>[4x]SNAMEPVSSWGNTSLVSVDPEIHDLIEKEKRRQCRGIELIASENFTSFAVIEALGSALTNKYSEGIPGNRYYGGNEFIDEIENLCRSRALEAFHCDPAAWGVNVQPYSGSPANFAAYTALLQPHDRIMGLDLPSGGHLTHGYYTSGGKKISATSIYFESLPYKVNFTTGYIDYDKLEEKALDFRPKLLICGGSAYPRDWDYARFRAIADKVGALLLCDMAHISGLVAAQEAANPFEYCDVVTTTTHKSLRGPRAGMIFYRKGPKPPKKGQPEGAVYDFEDKINFAVFPALQGGPHNHQIGALAVALKQANTPGFKVYAKQVKANAVALGNYLMSKGYQIVTNGTENHLVLWDLRPLGLTGNKVEKLCDLCSITLNKNAVFGDSSALAPGGVRIGAPAMTSRGLVEKDFEQIGEFLSRAVTLTLDIQKTYGKLLKDFNKGLVNNKDLDQLKADVEKFSASYEMPGFLMSEMKYKD

Serine hydroxymethyltransferase (SHMT) reversibly interconverts serine and tetrahydrofolate (THF) into glycine and 5,10-methylene-THF (5,10-meTHF). Next, we have obtained high resolution crystal structures of AtSHMT2 complexed with MTX and PTX, as well as of AtSHMT4-MTX complex. For clarity, in this work we divide THF, MTX, and PTX molecules into three moieties: (i) pteridine or its mimic (P-moiety); (ii) benzoyl (B-moiety); and (iii) glutamate (E-moiety).

In AtSHMT4, all four subunits within the crystal structure are in the external aldimine PLP-Ser form. In AtSHMT4, (chain D) N1 of pteridine-2,4-diamine (with sp3 hybridization) interacts with Nζ of Lys373, whereas exocyclic N2 binds to carbonyl O of Arg67. The pteridine ring is stacked with the side chain of Tyr68*, equivalent to Tyr111* in AtSHMT2. The B-moiety is shielded by Ile147, Tyr139, and Ala382, corresponding to Ile189, Tyr182, and Ala423 of AtSHMT2, respectively. The E-moiety interacts with the backbone amide of Ala382 and Oγ of Ser142. Despite most of the interacting residues being conserved in AtSHMT2 and AtSHMT4, positioning of the P-moiety of MTX is different. Therefore, it is striking to see that the P-moiety in AtSHMT4 structure is posed in the same plane but rotated 180° with respect to the IA-type in AtSHMT2. Consistently, the stacking Tyr68* has a conformation similar to that of the corresponding Tyr111* of AtSHMT2 in the IA-type, and not to the EA-type as expected. Variability is present in the E-moiety binding region, however, the residue that ensures positive charge of the loop (Lys145 in AtSHMT4 and Lys187 in AtSHMT2) is universally conserved.(1R,2R,3R,5Z,7E,14beta,17alpha)-2-(3-hydroxypropoxy)-9,10-secocholesta-5,7,10-triene-1,3,25-triol | C30 H50 O5 | 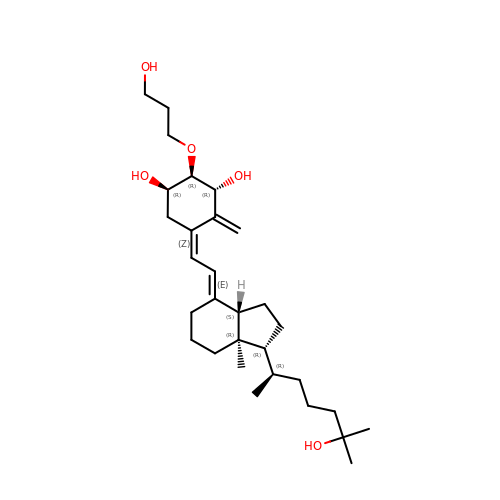FZEXGDDBXLBRTD-AYIMTCTASA-N> MNSNKDKIKVIKVFEAFAGIGSQFKALKNIARSKNWEIQHSGMVEWFVDAIVSYVAIHSKNFNPKIERLDRDILSISNDSKMPISEYGIKKINNTIKASYLNYAKKHFNNLFDIKKVNKDNFPKNIDIFTYSFPCQDLSVQGLQKGIDKELNTRSGLLWEIERILEEIKNSFSKEEMPKYLLMENVKNLLSHKNKKNYNTWLKQLEKFGYKSKTYLLNSKNFDNCQNRERVFCLSIRDDYLEKTGFKFKELEKVKNPPKKIKDILVDSSNYKYLNLNKYETTTFRETKSNIISRPLKNYTTFNSENYVYNINGIGPTLTASGANSRIKIETQQGVRYLTPLECFKYMQFDVNDFKKVQSTNLISENKMIYIAGNSIPVKILEAIFNTLEFVNNEE

M.MpeI is a prokaryotic CpG specific C5 cytosine DNA methyltransferase, and a good model for mammalian DNMT1, because of the same specificity. In contrast to most other DNA methyltransferases, M.MpeI and DNMT1 also unstack the CpG in the non-substrate strand, by additional amino acid intercalation (Trp and Lys in DNMT1, Phe in M.MpeI). Like other C5 methyltransferases, DNMT1 catalyzes methylation through the formation of a covalent protein-DNA intermediate resulting from the addition of an active site cysteine (of the so-called motif IV) to the cytosine C6 atom (with concomitant N3 protonation). Crystal structures of M.MpeI-DNA complexes capture the ‘in’ conformation of the active site loop for analogues with small or rotatable (5mZ) 5-substituents and its ‘out’ form for bulky 5-substituents.

The M.MpeI ‘in’ conformation has an inaccessible active site and probably traps the catalytically productive state. It is observed for 5FC, and surprisingly also for 5mZ containing DNA in complex with M.MpeI. In this form, Cys135 is poised for the nucleophilic attack on the C6 atom of the substrate base. The distances between the cysteine Sγ and the C6 carbon of the analogue are 2.9 Å for 5FC and 2.6 Å for 5mZ. The ‘in’ conformation is observed in the 5mZ complex despite the presence of the 5-methyl group. Steric conflict is in this case avoided due to the greater rotational freedom of 5mZ compared to the other bases. For the natural base cytosine and the other analogues, the N4 amino group hydrogen bonds with the side chain of Glu184, and a main-chain carbonyl oxygen of Phe133. The interactions fix the plane of the base. 5mZ, which lacks this amino group, is freer to rotate and therefore can avoid the steric clash between the methyl group and the active site loop in the ‘in’ conformation. SAH or a mixture of SAM and SAH is present in the complexes with the loop in the ‘in’ conformation.> MESKRNKPGKATGKGKPVGDK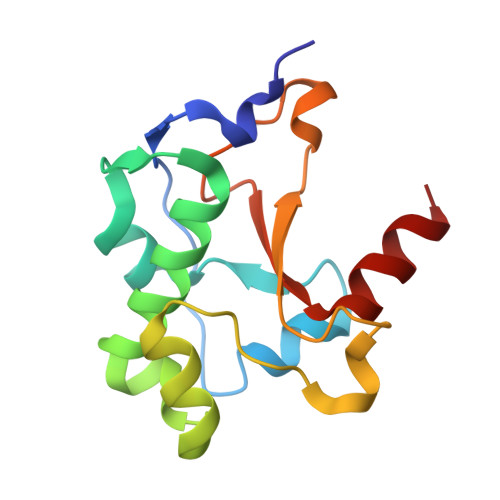WLDDAGKDSGAPIPDRIADKLRDKEFKSFDDFRKAVWEEVSKDPELSKNLNPSAKSSVSKGYSPFTPKNQQVGGRKVYELHHDKPISQGGEVYDMDNIRVTTPKRHIDIHRGK>[12x]MAQVQQLTPAQQAALRNQQAMAANLQARQIVLQQSYPVIQQVETQTFDPANRSVFDVTPANVGIVKGFLVKVTAAITNNHATEAVALTDFGPANLVQRVIYYDPDNQRHTETSGWHLHFVNTAKQGAPFLSSMVTDSPIKYGDVMNVIDAPATIAAGATGELTMYYWVPLAYSETDLTGAVLANVPQSKQRLKLEFANNNTAFAAVGANPLEAIYQGAGAADCEFEEISYTVYQSYLDQLPVGQNGYILPLIDLSTLYNLENSAQAGLTPNVDFVVQYANLYRYLSTIAVFDNGGSFNAGTDINYLSQRTANFSDTRKLDPKTWAAQTRRRIATDFPKGVYYCDNRDKPIYTLQYGNVGFVVNPKTVNQNARLLMGYEYFTSRTELVNAGTISTT;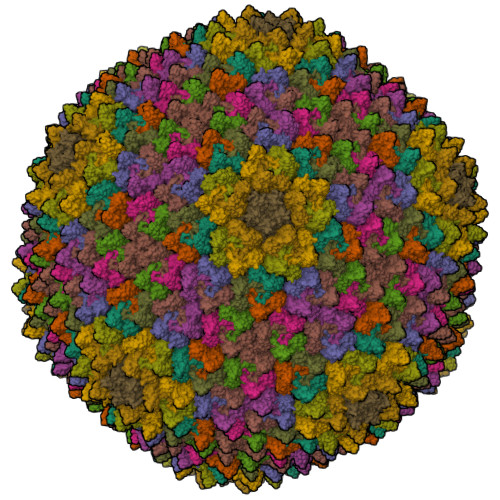> ALINPQFPYAGPVPIPGPAPTETMPLLNYRVEGRIAGIQQARQFMPFLQGPHRAVAEQTYHAIGTGIQMGQTFNQPLINTQEG;> MNVNNPNQMTVTPVYNGCDSGEGPQSVRGYFDAVAGENVKYDLTYLADTQGFTGVQCIYIDNAENDGAFEIDVEETGQRIKCPAGKQGYFPLLVPGRAKFVARHLGSGKKSVPLFFLNFTIAQGVW;> MDKKKLLYWVGGGLVLILIWLWFRNRPAAQVASNWEGPPYMTYNQPQAGSVTLPVAGYTSPSPTLPNRNRSCGCNPAVSAAMAQGADLASKLTDSITSQLNDYASSLNDYLASQAGV>GHMLGSILPFNEETADRVSAYCEKNSHGIPDALVEHWEWTRTRFPDADKMSSRLQGSWMIFTARDRKPKRILEIGCYSGYSALAWYEGTRDTKAEIVTLEYSPKMIAASREAFKKYGVGDRVKLIEGPAENTLKTLEGEFDLIFVDANKDGYAGYVKTILDQGLLSANGIILCDN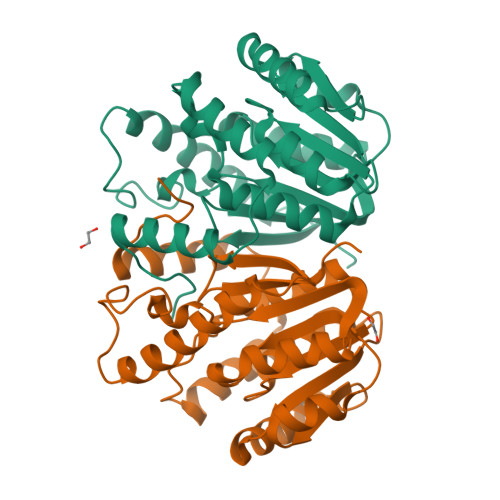VFARGLTIGPDCAPWLNDHVRPYWNGCGQALDKFSAGLMEDPRIDVLLLPVFDGVTQIRWKDGAQRA[2x]> IVGGQECKDGECPWQALLINEENEGFCGGTILSEFYILTAAHCLYQAKRFKVRVGDRNTEQEEGGEAVHEVEVVIKHNRFTKETYDFDIAVLRLKTPITFRMNVAPACLPERDWAESTLMTQKTGIVSGFGRTHEKGRQSTRL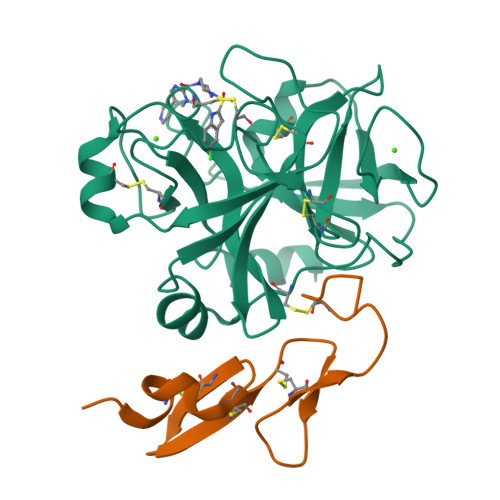KMLEVPYVDRNSCKLSSSFIITQNMFCAGYDTKQEDACQGDSGGPHVTRFKDTYFVTGIVSWGEGCARKGKYGIYTKVTAFLKWIDRSMK;> KDGDQCETSPCQNQGKCKDGLGEYTCTCLEGFEGKNCELFTRKLCSLDNGDCDQFCHEEQNSVVCSCARGYTLADNGKACIPTGPYPCGKQTLER> 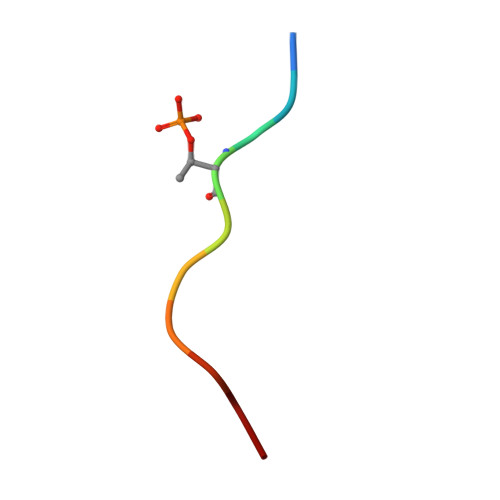SDATEGHDED> GSPGISGGGGGILDSMDVVSLDKPFMYFEEIDNELDYEPESANEVAKKLPYQGQLKLLLGELFFLSKLQRHGILDGATVVYIGSAPGTHIR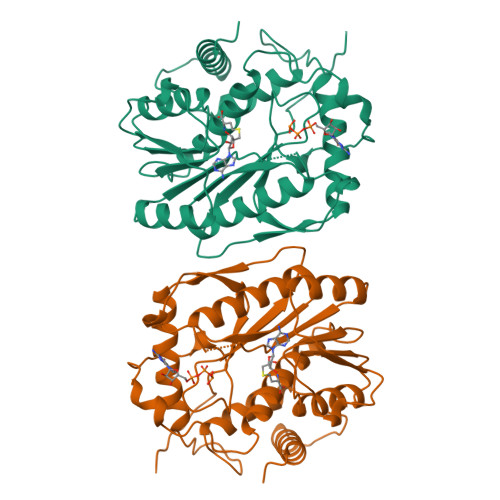YLRDHFYNLGVIIKWMLIDGRHHDPILNGLRDVTLVTRFVDEEYLRSIKKQLHPSKIILISDVRSKRGGNEPSTADLLSNYALQNVMISILNPVASSLKWRCPFPDQWIKDFYIPHGNKMLQPFAPSYSAEMRLLSIYTGENMRLTRVTKSDAVNYEKKMYYLNKIVRNKVVVNFDYPNQEYDYFHMYFMLRTVYCNKTFPTTKAKVLFLQQSIFRFLNIPTTSTEKVSHE5-fluoronicotine 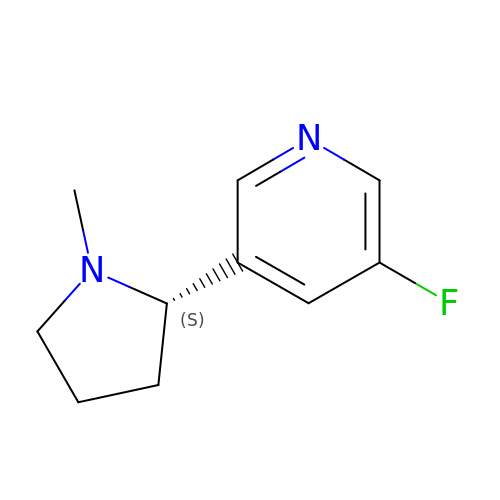| C10 H13 F N2 | WEACEDDYURLEPK-JTQLQIEISA-N>MRGSHHHHHHGTGENLYFQGGSPEQMAEEIR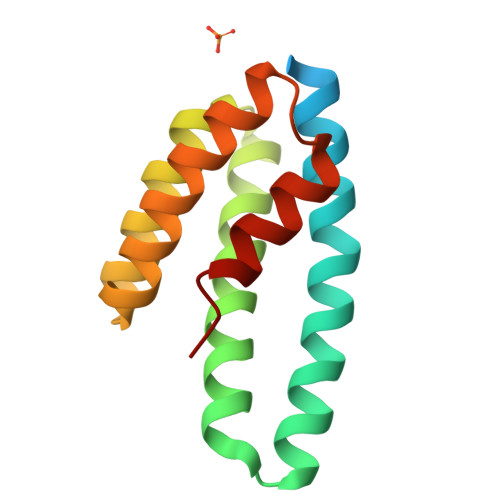QALEKILKQLENEIEIARNAGDDEREDRYRIAYLAALEAYRLLAEGVRIPEAVQRAAAYLASMGYPHYAELFRAKGEELVKRLLEGKVTGEEFARQLVFYPAQAV[2x]> HHHHHHFNLPPGNYKKGGTVDGTRDRSDTHIQFQISPEGNGEVLLKSTETGQYLRINPDGTVDGTRDRSDTHIQFQISPE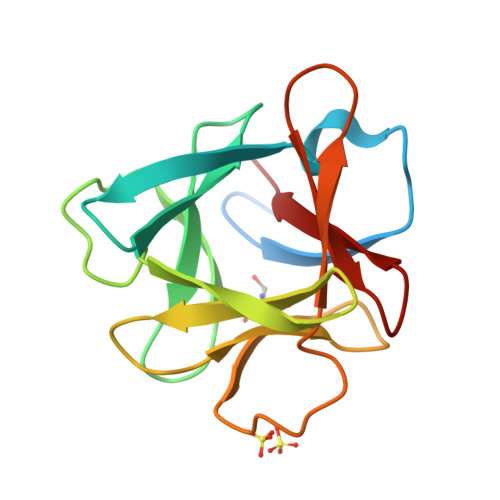GNGEVLLKSTETGQYLRINPDGTVDGTRDRSDTHIQFQISPEGNGEVLLKSTETGQYLRINP>EVLTGGHSVSAPQENRIYVMDSVFMHLTESRVHVYDYTNGKFLGMVPTAFNGHVQVSNDGKKIYTMTTYHERITRGKRSDVVEVWDADKLTFEKEISLPPKRVQGLNYDGLFRQTTDGKFIVLQNASPATSIGIVDVAKGDYVEDVTAAAGCWSVIPQPNRPRSFMTICGDGGLLTINLGEDGKVASQSRSKQMFSVKDDPIFIAPALDKDKAHFVSYYGNVYSADFSGDEVKVDGPWSLLNDEDKAKNWVPGGYNLVGLHRASGRMYVFMHPDGKEGTHKFPAAEIWVMDTKTKQRVARIPGRDALSMTIDQQRNLMLTLDGGNVNVYDISQPEPKLLRTIEGAAEASLQVQFHPV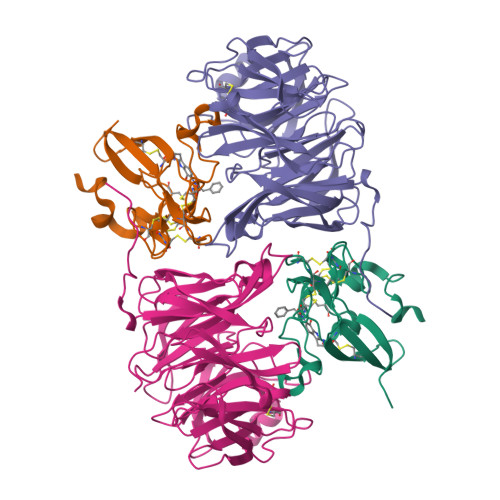GGT[2x];>[2x]HISLNPDLANEDEVNSCDYWRHCAVDGFLCSCCGGTTTTCPPGSTPSPISWIGTCHNPHDGKDYLISYHDCCGKTACGRCQCNTQTRERPGYEFFLHNDVNWCMANENSTFHCTTSVLVGLAKN> GPLQYKDLKIDIKTSPPPECINDALQAVDSQEVRDY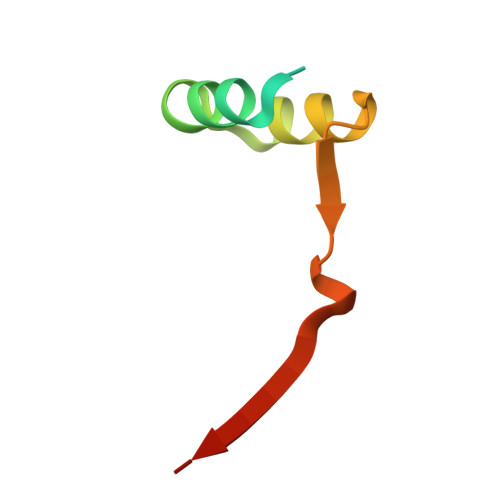CEKKGWIVNITSQVQTERNINR> ALFDYNATGDTEFDSPAKQGWMQDNTNNGSGVLTNADGMPAWLVQGIGGRAQWTYSLSTNQHAQASSFGWRMTTEMKVLSGGMITNYYANGTQRVLPIISLDSSGNLVVEFEGQTGRTVLATGTAATEYHKFELVFLPGSNPSASFYFDGKLIRDNIQPTASKQNMIVWGNGSSNTDGVAAYRDIKFEIQGDVIFRGPDRIPSIVASSVTPGVVTAFAEKRVGGGDPGALSNTNDIITRTSRDGGITWDTELNLTEQINVSDEFDFSDPRPIYDPSSNTVLVSYARWPTDAAQNGDRIKPWMPNGIFYSVYDVASGNWQAPIDVTDQVKERSFQIAGWGGSELYRRNTSLNSQQDWQSNAKIRIVDGAANQIQVADGSRKYVVTLSIDESGGLVANLNGVSAPIILQSEHAKVHSFHDYELQYSALNHTTTLFVDGQQITTWAGEVSQENNIQFGNADAQIDGRLHVQKIVLTQQGHNLVEFDAFYLAQQTPEVEKDLEKLGWTKIKTGNTMSLYGNASVNPGPGHGITLTRQQNISGSQNGRLIYPAIVLDRFFLNVMSIYSDDGGSNWQTGSTLPIPFRWKSSS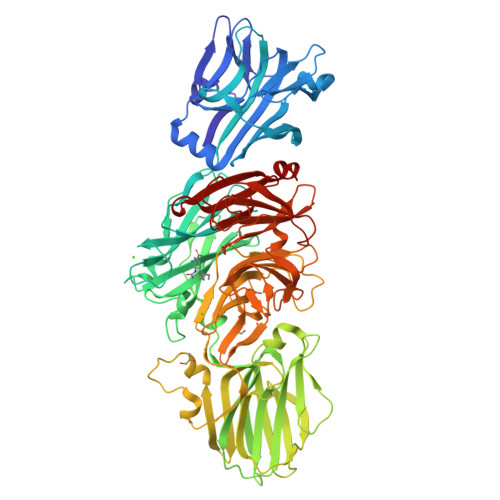ILETLEPSEADMVELQNGDLLLTARLDFNQIVNGVNYSPRQQFLSKDGGITWSLLEANNANVFSNISTGTVDASITRFEQSDGSHFLLFTNPQGNPAGTNGRQNLGLWFSFDEGVTWKGPIQLVNGASAYSDIYQLDSENAIVIVETDNSNMRILRMPITLLKQKLTLSQN rotundine | C21 H25 N O4 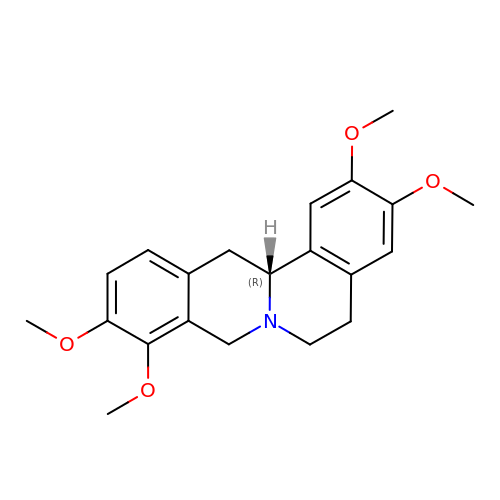| AEQDJSLRWYMAQI-QGZVFWFLSA-N> PDQFRAIIESPEGAGHVGYQYRRNTGSTMRMVSDVLDERVSLWDFHCDPSGNVIQPGPNVDSRQYLQAAIDYVSSNGGGTITIPAGYTWYLGSYGVGGIAGHSGIIQLRSNVNLNIEGRIHLSPFFDLKPFQVFVGFDNGDPASSGNLENCHIYGHGVVDFGGYEFGASSQLRNGVAFGRSYNCSVTGITFQNGDVTWAITLGWNGYGSNCYVRKCRFINLVNSSVNANHSTVYVNCPYSGVESCYFSMSSSFARNIACSVELHQHDTFYRGSTVNGYCRGAYVVMHAAEAAGAGSYAYNMQVENNIAVIYGQFVILGSDVTATVSGHLNDVIVSGNIVSIGERAAFSAPFGAFIDIGPDNSGASNVQDIQRVLVTGNSFYAPANITDSAAITLRANLNGCTFIANNFDCRYMVYNAPGTTSPVVQNLVWDKSNVIGGTHANQRAGQNLFDMQFASVVNSTIEVQLSCEDLSMFSCILFPASCQLSYSKITVDSAWTKSMSNTAVFEGNQQAGANVYVSYPATVNLTSYNTQGAVPFFSTDTNYAWVTSAYSLSINENLDFSPPATYTNKAN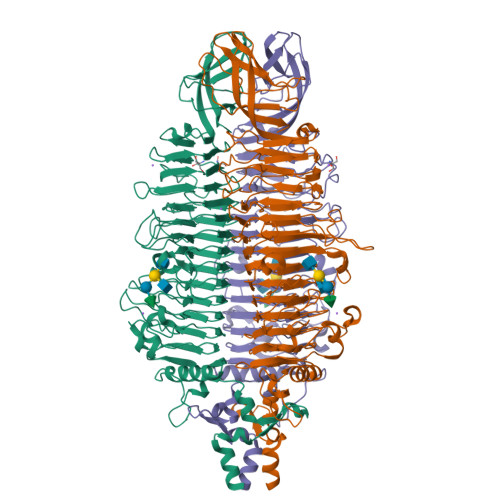GQLVGVGYNEIGGVRSVSVRLMLQRQV>MNPPTTTTTTTRTIRAPKVQLTPNSATRRRRNRRRRRPAAAIAGPLSIQPSSINRRMVSRVTRRSAVVTAAGLAWLRQYLNPMGPDTTSVTGYPDGS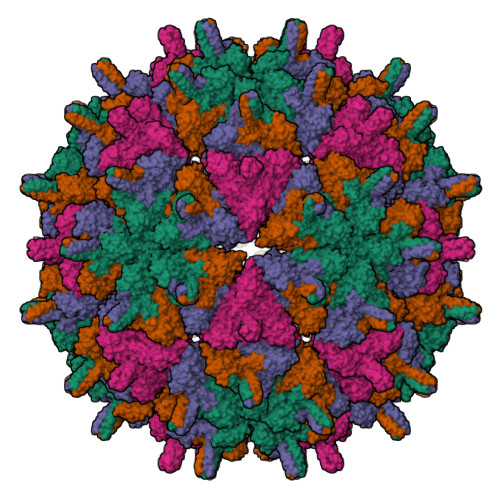AVTTCIADYSNTFNVSFPPREALYCTGSSSSEKPTLVDADNYAKIDKWSNYDITLCVLALPMLRNVVMLRLYPHTPTAFALTEQTPNFPQRFPNWSVYSADGTRFNNGDEPGYLQSYVYLPNVDKHLSAARGYRLLSRGITGIFSAPALETQGFVTACQYLAEGSIQSQSIKSDAVRSVTVNSDGTVKNVESSSQTVSSMPRYVFPLDGDNCAPSSLTETYHQAYQSKATDGFYMPVLSSSRDNPFHPPQPRAIAVYGSFLARGCLDPVSEAHEADGPTHDIYRLNVADDVAPLFNTGVVWFEGISPKFSLKLKTRTVLQYIPTSGSVLANFTRHEPTYDQIALDAADRLRNLMPHAYPAAYNDWGWLGDLLDSAISMLPGVGTVYNIAKPLIKPAWNWLGNKVSDFFGNPVARDGDIFFDAK[4x]> MRKELVFVLLALFLCAGCNGNKKKMNGEHDL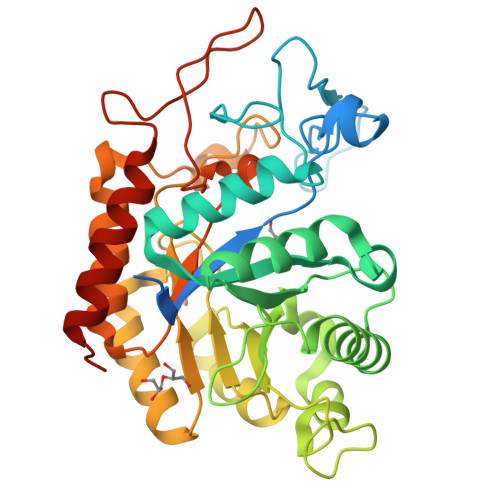DAANITLDDHTISFYYNWYGNPSVDGEMKHWMHPIALAPGHSGDVGAISGLNDDIACNFYPELGTYSSNDPEIIRKHIRMHIKANVGVLSVTWWGESDYGNQSVSLLLDEAAKVGAKVCFHIEPFNGRSPQTVRENIQYIVDTYGDHPAFYRTHGKPLFFIYDSYLIKPAEWAKLFAAGGEISVRNTKYDGLFIGLTLKESELPDIETACMDGFYTYFAATGFTNASTPANWKSMQQWAKAHNKLFIPSVGPGYIDTRIRPWNGSTTRDRENGKYYDDMYKAAIESGASYISITSFNEWHEGTQIEPAVSKKCDAFEYLDYKPLADDYYLIRTAYWVDEFRKARSASEDVQ;> MRKELVFVLLALFLCAGCNGNKKKMNGEHDLDAANITLDDHTISFYYNWYGNPSVDGEMKHWMHPIALAPGHSGLVGAISGLNDDIACNFYPELGTYSSNDPEIIRKHIRMHIKANVGVLSVTWWGESDYGNQSVSLLLDEAAKVGAKVCFHIEPFNGRSPQTVRENIQYIVDTYGDHPAFYRTHGKPLFFIYDSYLIKPAEWAKLFAAGGEISVRNTKYDGLFIGLTLKESELPDIETACMDGFYTYFAATGFTNASTPANWKSMQQWAKAHNKLFIPSVGPGYIDTRIRPWNGSTTRDRENGKYYDDMYKAAIESGASYISITSFNEWHEGTQIEPAVSKKCDAFEYLDYKPLADDYYLIRTAYWVDEFRKARSASEDVQ>[2x]GGSARERDTSRRLLAEKEREMAEMR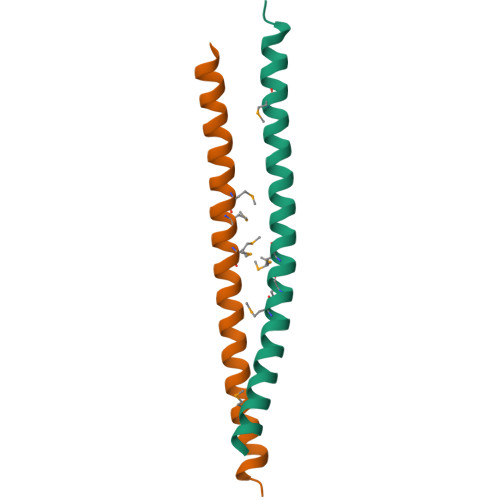ARMQQQLDEYQELLDIKLALDMEIHAYRKLLEGEEERLRLSPSPTSQRS> HHHHSQDGGAYSDERQDLDQTIAEVSKELKLKLLIVENFIPRDVSERIKERAEWNEDSFEWNVNAFQSTSSNSSTPLNNTIEVNEDGVFTRSSGADSGVSVSGGNGTPATSQFLDKRLVATPGCRRPMSMCERMLVETAREQFGAQRRPPISGSGSFVEATIPEETIRFCGENVVVFSALERFVPEVTDSDPSTFSNSMMMSARRPSIENLTIDASKVLVPILNQSTMILKNSKNGQARNDTMPPNGSMRRSQN;> EDHQRQVEAMLDDIRQLRKELLLNIAIIDEYIPVEHVELIEKYVSWSEEHGDWQLKAIAYTGNNMRASAPPAKKEFSNNNQTVPMYYSYRADLGASTAEHRPRTSSKKHRASIRLQQLLT;> ELGKIDEYIECFYGETSVEKNKGAVALYELSKNPQNLTQLVNNETLMMALARVFREDWKKHFEVGTNIMNLFVNISKFSCLHGILLHHKIGTLCVNAMEHETKRYDFWIAEMKKTDQETLRKLKTAIRKQAMLLAACVTFLTNLATDISVELKMVRRNLVALLVKCLQMSSESTSSLTTATIKFLLKLSIFDENKIVMEQNGTIEKLLKLFPIQDPELRKAVIMLLFNFSFDSKNLPKMVNGGLVPHMASLLDSDTKALNMMYLLSCNDDAKAMLAYTDAIKLLMKDVLSGTGSEVTKAVLLNICLEKRNAQLVCGQRGQGLDLLMEMSINSRDLMLIKVVRAISSHEGATQNMFLKWIETLIGIAKNEGADNSESKSSFGLECMGTVAELKVAPWAKIIQSENLVPWMKTQLQEGIDESEEVTVLRDIKPLQLQIVIACGTMARQLDAARLLAPLIDTFVQLLQSCQIDDEFVVQLLYVFLQFLKHKELSARLMTQDSALGAHMIDLMHDANAVVREVCDNALLIMGEHSKEWAKRIAGERFKWHNAQWLEMVERDDSE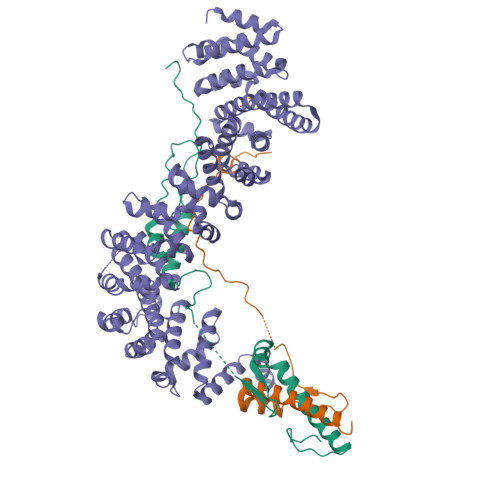FVDYDDEDFGADLKFDHYDDGFDMNEPLF> SNAMRVIVTEYQPAWVEQFEEEAQALKQILKENCLKVEHIGSTSVPNLAAKPIIDFLVIVEEIEKVDLLQWEFERIGYEYMGEFGLSGRRYLRKGPIKRTHHVHIY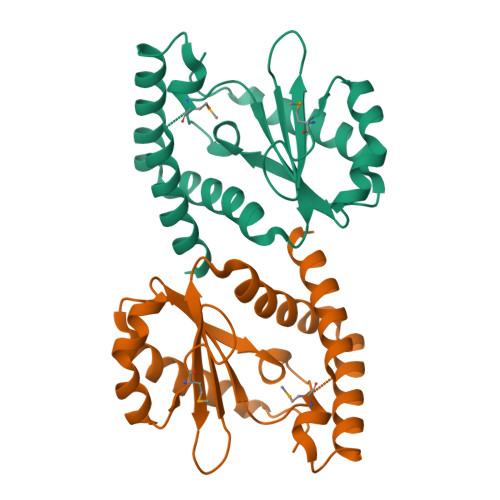QFDNTQEILRHLAFRNYLRENPAIATTYGTLKKQLAQAHPDSIDKYMDGKDAFIKKIEKEALKKYWE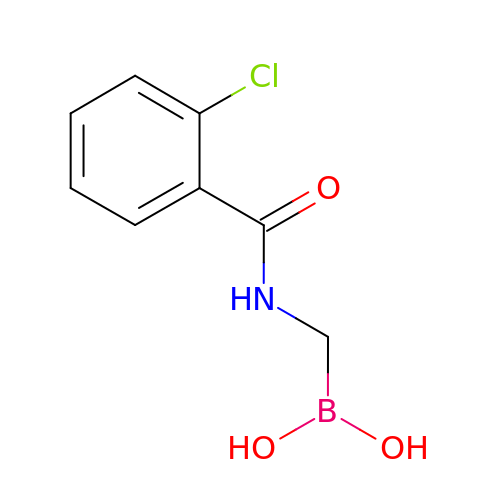{[(2-chlorobenzoyl)amino]methyl}boronic acid | C8 H9 B Cl N O3 | LXIUYRUEMMFAQV-UHFFFAOYSA-N> MFKAPPILPPHLLQVILNKDTGISCDP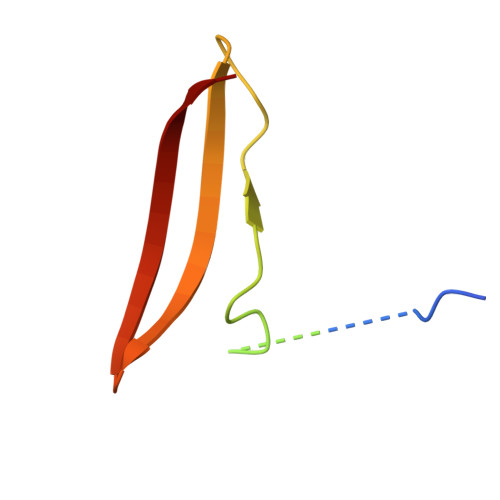ALLPEPNHVMLNHLYALSIKDGVMVLSATHRYKKKYVTTLLYKPI> MSDLDTFTFIPLHIDPKSKAISAAPNALGTPSANKALETELAALNALHRALHTQIEGPIPVPPPPVPVNPKRSANINKLRESGNAEYRKQRYGDAIKLYTLGLQMALTRPAWEPAGLVRDEIHQLYSNRAQAYMQLGQWPEAAADAECSVEAKRQGNAK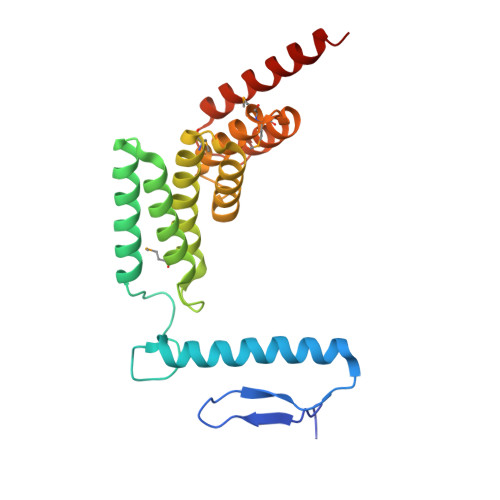AWYRRGKCLMEMRRLQEAREWVARGLEFEGEEKELAELLKEIDSKLAAEKASRDA> GELPEVETVRRELEKRIVGQKIISIEATYPRMVLTGFEQLKKELTGKTIQGISRRGKYLIFEIGDDFRLISHLRMEGKYRLATLDAPREKHDHLTMKFADGQLIYADVRKFGTWELISTDQVLPYFLK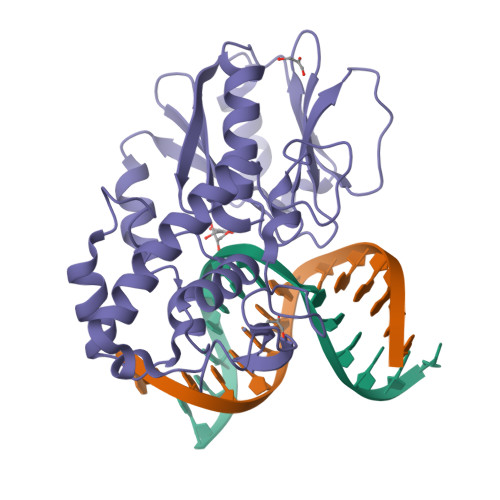KKIGPEPTYEDFDEKLFREKLRKSTKKIKPYLLEQTLVAGLGNIYVDEVLWLAKIHPEKETNQLIESSIHLLHDSIIEILQKAIKLGGSSIRTYSALGSTGKMQNELQVYGKTGEKCSRCGAEIQKIKVAGRGTHFCPVCQQK>GPGKTDSSFIMDSDPRRCMRHHYVDSISHPLYKCSSKMVLLARCEGHCSQASRSEPLVSFSTVLKQPFRSSCHCCRPQTSKLKALRLRCSGGMRL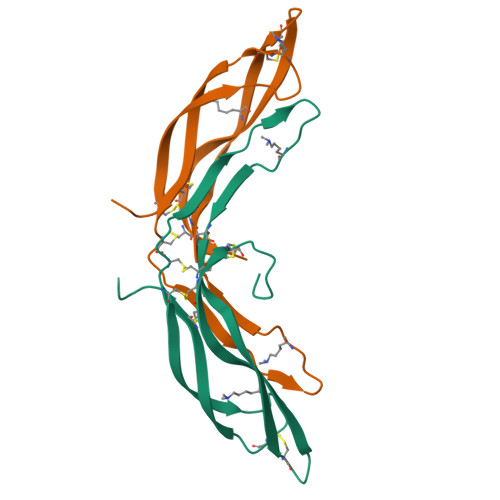TATYRYILSCHCEECNSGTETSQVAPA[4x]>[2x]MIDERDKIILEILEKDARTPFTEIAKKLGISETAVRKRV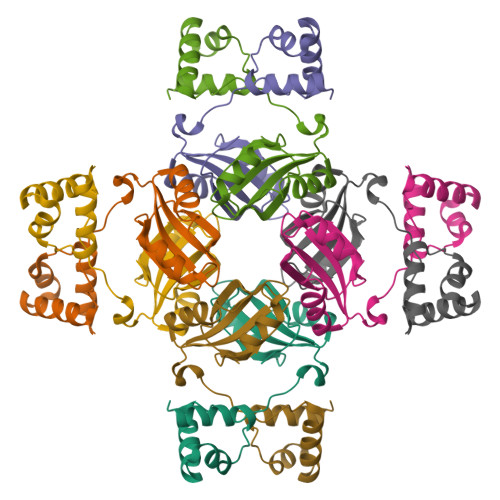KALEEKGIIEGYTIKINPKKLGYSLVTITGVDTKPEKLFEVAEKLKEYDFVKELYLSSGDHMIMAVIWAKDGEDLAEIISNKIGKIEGVTKVCPAIILEKLK>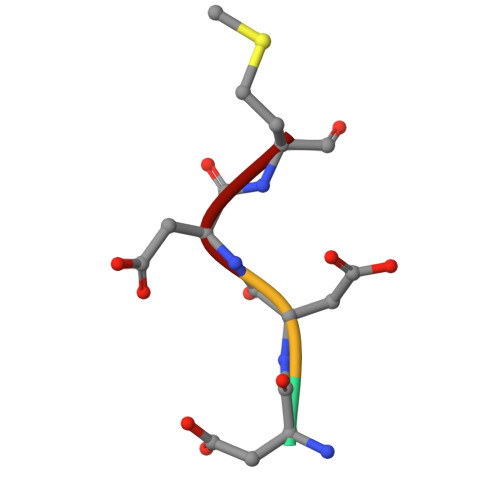 DDDM>[2x]MTTTITEMSATIVDLPSRRPHKFAATTMHHQSIVLVRVRDSDGGEGIGEAVTPGGPWWGGESVETIKTIIDQYLAPVIIGRDPSTIGVASQSMDGLVFGNSVAKAAIETALWDDRERRSRIPVSDLLGGLRRKRIPITWAFSAGSASDLIDEAAQKLDVGHRSFKFKMGAEPADTDSRRVLDVLECIPDECAVI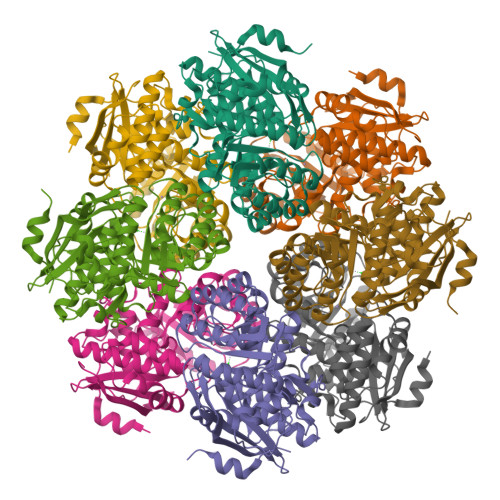VDPNGRWSELEAHRWLPILADAGVTVAEQPIARWNTDGLARLRDKLSIPIMADESVTTVQQAIALADAGAVSAFAIKIPKSGGLSRAREIAAIAEASGLACFGAATPESSVMGAISAQLYGTMPDLSVGCELFGPGLLIDEVVTEPLKYDRGELLIPTGPGSGVNLDEERLRKYSRD> MLGLKTSIIGRRVIYFQEITSTNEFAKTSYLEEGTVIVADKQTMGHGALNRKWESPEGGLWLSIVLSPKVPQKDLPKIVFLGAVGVVETLKEFSIDGRIKWPNDVLVNYKKIAGVLVEGKGDKIVLGIGLNVNNKVPNGATSMKLELGSEVPLLSVFRSLITNLDRLYLNFLKNPMDILNLVRDNMILGVRVKILGDGSFEGIAEDIDDFGRLIIRLDSGEVKKVIYGDVSLRF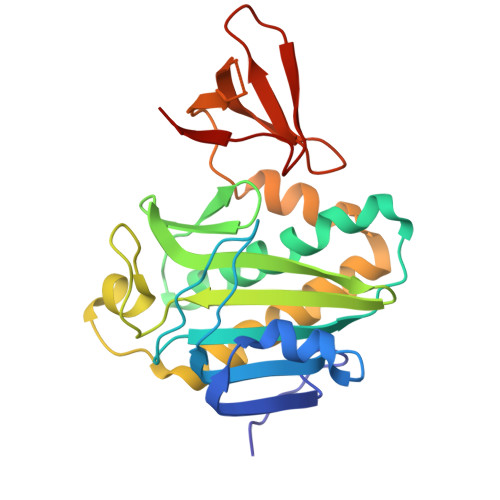L> MKLKTTLFGNVYQFKDVKEVLAKANELRSGDVLAGVAAASSQERVAAKQVLSEM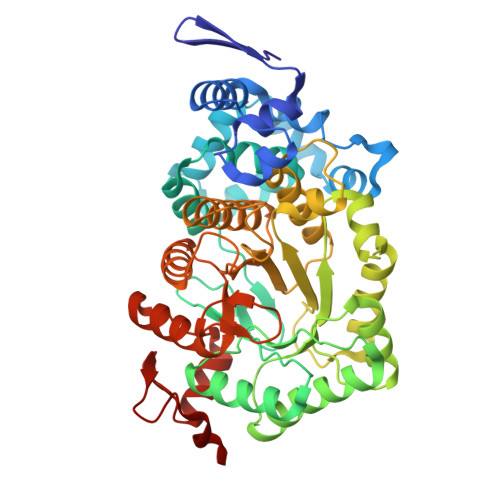TVADIRNNPVIAYEDDCVTRLIQDDVNETAYNQIKNWSISELREYVLSDETSVDDIAFTRKGLTSEVVAAVAKICSNADLIYGAKKMPVIKKANTTIGIPGTFSARLQPNDTRDDVQSIAAQIYEGLSFGVGDAVIGVNPVTDDVENLSRVLDTIYGVIDKFNIPTQGCVLAHVTTQIEAIRRGAPGGLIFQSICGSEKGLKEFGVELAMLDEARAVGAEFNRIAGENCLYFETGQGSALSAGANFGADQVTMEARNYGLARHYDPFIVNTVVGFIGPEYLYNDRQIIRAGLEDHFMGKLSGISMGCDCCYTNHADADQNLNENLMILLATAGCNYIMGMPLGDDIMLNYQTTAFHDTATVRQLLNLRPSPEFERWLESMGIMANGRLTKRAGDPSLFF>[12x]MSSAIKEVQGAPVKWVTNWTPEAIRGLVDQEKGLLDPRIYADQSLYELELERVFGRSWLLLGHESHVPETGDFLATYMGEDPVVMVRQKDKSIKVFLNQCRHRGMRICRSDAGNAKAFTCSYHGWAYDIAGKLVNVPFEKEAFCDKKEGDCGFDKAEWGPLQARVATYKGLVFANWDVQAPDLETYLGDARPYMDVMLDRTPAGTVAIGGMQKWVIPCNWKFAAEQFCSDMYHAGTTTHLSGILAGIPPEMDLSQAQIPTKGNQFRAAWGGHGSGWYVDEPGSLLAVMGPKVTQYWTEGPAAELAEQRLGHTGMPVRRMVGQHMTIFPTCSFLPTFNNIRIWHPRGPNEIEVWAFTLVDADAPAEIKEEYRRHNIRNFSAGGVFEQDDGENWVEIQKGLRGYKAKSQPLNAQMGLGRSQTGHPDFPGNVGYVYAEEAARGMYHHWMRMMSEPSWATLKP;>[12x]MTNPSPHFFKTFEWPSKAAGLELQNEIEQFYYREAQ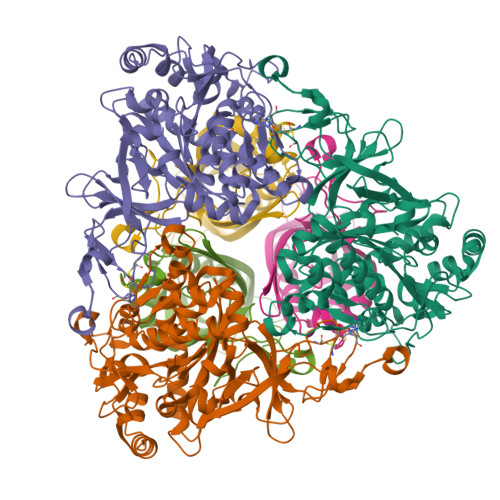LLDHRAYEAWFALLDKDIHYFMPLRTNRMIREGELEYSGDQDLAHFDETHETMYGRIRKVTSDVGWAENPPSRTRHLVSNVIVKETATPDTFEVNSAFILYRNRLERQVDIFAGERRDVLRRADNNLGFSIAKRTILLDASTLLSNNLSMFF>MNLPTAQEVQGLMARYIELVDVGDIEAIVQMYADDATVEDPFGQPPIHGREQIAAFYRQGLGGGKVRACLTGPVRASHNGCGAMPFRVEMVWNGQPCALDVIDVMRFDEHGRIQTMQAYWSEVNLSVREPQLVP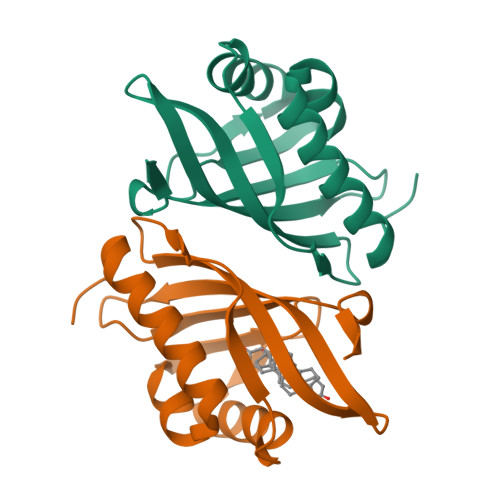R[2x]>MKLTPKELDKLMLHYAGELARKRKEKGIKLNYVEAVALISAHIMEEARAGKKTAAELMQEGRTLLKPDDVMDGVASMIHEVGIEAMFPDGTKLVTVHTPIEANGKLVPGELFLKNEDITINEGKKAVSVKVKNVGDRPVQIGSHFHFFEVNRCLDFDREKTFGKRLDIASGTAVRFEPGEEKSVELIDIGGNRRIFGFNALVDRQADNESKKIALHRAKERGFHGTKSDDNYVKTIKE[12x];>MKKISRKEYVSMYGPTTGDKVRLGDTDLIAEVEHDYTIYGEELKFGGGKTLREGMSQSNNPSKEELDLIITNALIVDYTGIYKADIGIKDGKIAGIGKGGNKDMQDGVKNNLSVGPATEALAGEGLIVTAGGIDTHIHFISPQQIPTAFASGVTTMIGGGTGPADGTNATTITPGRRNLKWMLRAAEEYSMNLGFLAKGNTSNDASLADQIEAGAIGFKIHEDWGTTPSAINHALDVADKYDVQVAIHTDTLNEAGCVEDTMAAIAGRTMHTFHTEGAGGGHAPDIIKVAGEHNILPASTNPTIPFTVNTEAEHMDMLMVCHHLDKSIKEDVQFADSRIRPQTIAAEDTLHDMGIFSITSSDSQAMGRVGE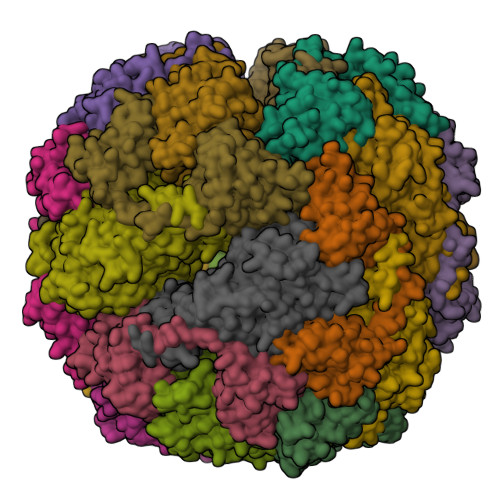VITRTWQTADKNKKEFGRLKEEKGDNDNFRIKRYLSKYTINPAIAHGISEYVGSVEVGKVADLVLWSPAFFGVKPNMIIKGGFIALSQMGDANASIPTPQPVYYREMFAHHGKAKYDANITFVSQAAYDKGIKEELGLERQVLPVKNCRNITKKDMQFNDTTAHIEVNPETYHVFVDGKEVTSKPANKVSLAQLFSIF[12x]>EGPIDKLKTPEDVPNDPLPLISDFEWSTLDIDDNLQLDELYKLLYDNYVEDIDATFRFKYSHEFFQWALKPPGWRKDWHVGVRVKSTGKLVAFIAATPVTFKLNKSNKVIDSVEINFLCIHKKLRNKRLAPVLIKEITRRVNKQNIWQALYTGGSILPTPLTTCRYQHRPINWSKLHDVGFSHLPPNQTKSSMVASYTLPNNPKLKGLRPMTGKDVSTVLSLLYKYQERFDIVQLFTEEEFKHWMLGHDENSDSNVVKSYVVEDENGIITDYFSYYLLPFTVLDNAQHDELGIAYLFYYASDSFEKPNYKKRLNELITDALITSKKFGVDVFNCLTCQDNTYFLKDCKFGSGDGFLNYYLFNYRTFPMDGGIDKKTKEVVEDQTSGIGVVLL[2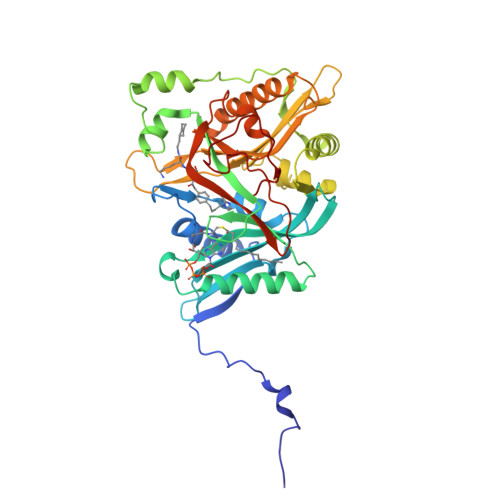x]>[4x]MRGSHHHHHHGIHMNSLIKENMRMMVVMEGSVNGYQFKCTGEGDGNPYMGTQTMRIKVVEGGPLPFAFDILATSFMYGSKTFIKHTKGIPDFFKQSFPEGFTWE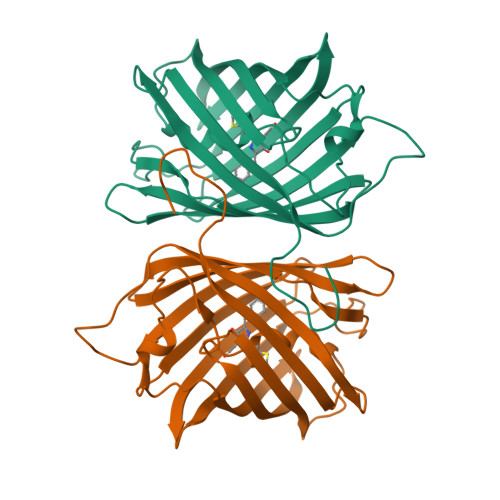RVTRYEDGGVFTVMQDTSLEDGCLVYHAKVTGVNFPSNGAVMQKKTKGWEPSTEMLYPADGGLRGYCQMALNVDGGGYLFCSFETTYRSKKTDENFKMPGFHFVDHRLERLEESDKEMFVVQHEHAVAKFCDLPSKLGRL>[5x]MPVAGSELPRRPLPPAAQERDAEPRPPHGELQYLGQIQHILRCGVRKDDRTGTGTLSVFGMQARYSLRDEFPLLTTKRVFWKGVLEELLWFIKGSTNAKELSSKGVKIWDANGSRDFLDSLGFSTREE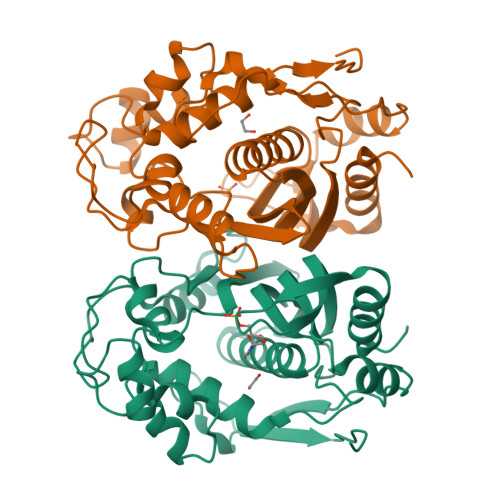GDLGPVYGFQWRHFGAEYRDMESDYSGQGVDQLQKVIDTIKTNPDDRRIIMCAWNPRDLPLMALPPCHALCQFYVVNSELSCQLYQRSGDMGLGVPFNIASYALLTYMIAHITGLKPGDFIHTLGDAHIYLNHIEPLKIQLQREPRPFPKLRILRKVEKIDDFKAEDFQIEGYNPHPTIKMEMAV>[2x]GSHMHTLYAPGGYDIMGYLIQIMNRPNPQVELGPVDTSCALILCDLKQKDTPIVY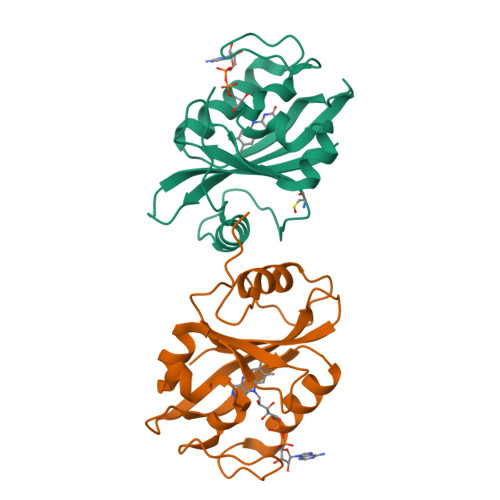ASEAFLYMTGYSNAEVLGRNCRFLQSPDGMVKPKSTRKYVDSNTINTMRKAIDRNAEVQVEVVNFKKNGQRFVNFLTMIPVRDETGEYRYSMGFQCETE>[2x]RGAEFTRLPVSWTVNPRDAANARAAWKTLSAYHRGKPKSSRKLHVVYVTFKDRPALEGYRERYDHILKNIQAYYADQMQANGFPPLTFQLDLDERGKLVIHDAYVDKPMSEMSVQSSGPVSREAARKVLASKGIDIEKEHVLVVCQLPDGVGPYYGGGFSHQGTGWTCDQEGLDPASFLDTEMMQGGRFKVTRGKNATIYIGGTAHELGHSFGLPHTGDGWNYPDAGASLMGHGNSTYGDELRHEGKGAYLAPTDALKLASVPLFNGVETELPADASFGRMLGKYVPGSFERLEAIPVKDGLRLKGRVHLTRPAYGIVAHLDPPGGSDYDSNAVGASLDEKGEFDLTICRPGYKGGFIEMRVAVLNCDSTRSMITLPVWMDARGTKAPSLAQIVYFGDVQNLWIRGRTEEARKALAEVERRHGSRSEVKEWLPVWKRALGR

The uncharacterized protein AMUC_1438 is encoded by a gene that was previously shown to be upregulated when the bacterium is grown on mucin. Here, we provide structural and functional support for the assignment of AMUC_1438 as a unique O-glycopeptidase with mucin-degrading capacity. Structural, kinetic, and mutagenic analyses point to a metzincin metalloprotease catalytic motif but with an active site that specifically recognizes a GalNAc residue α-linked to serine or threonine (i.e., the Tn-antigen). The enzyme catalyzes hydrolysis of the bond immediately N-terminal to the glycosylated residue.

We were unable to generate crystals of FL, but we were able to determine the structure of ALTL to 2.5 Å resolution. In this case, the last 18 amino acids in the two molecules in asymmetric unit were missing. The last ∼60 C-terminal amino acids that could be modeled, and which correspond to the missing residues in the ALT structure, comprised a three α-helix bundle resembling the Found In Various ARchitectures (FIVAR) domains observed as linkers in the ZmpB O-glycopeptidase from Clostridium perfringens. However, the relative orientations of the α-helical linker domain and the catalytic domain in the ALTL structure differ from the FL model, with the α-helical linker being packed more closely against the β-sandwich domain in ALTL than in the FL model. Indeed, the conformation observed in ALTL seems unlikely in the full-length enzyme as the position of the α-helical linker domain would likely result in clashes between the CBM-like domain, if it were present, and the rest of the protein. Toward providing support for the conformation observed in the FL model compared with the ALTL structure, we employed hydrogen-deuterium exchange mass spectrometry (HDX-MS) on both proteins. Most relevant to the FL model, however, is the increased exchange in the last two β-strands of the β-sandwich domain and the initial 1 to 2 turns of the first α-helix in the α-helical linker domain. In the ALTL crystal structure, these secondary structures are shielded from solvent by packing of the α-helical linker against the β-sandwich domain. In the FL model, however, the α-helical linker is peeled away from the β-sandwich domain, thus exposing the protein regions in FL that were observed to exchange more readily. Therefore, the HDX-MS results are consistent with conformation of the FL model.> GSHMARENEMDENLEQVSGIIGNLRHMALDMGNEIDTQNRQIDRIMEKADSNKTRIDEANQRA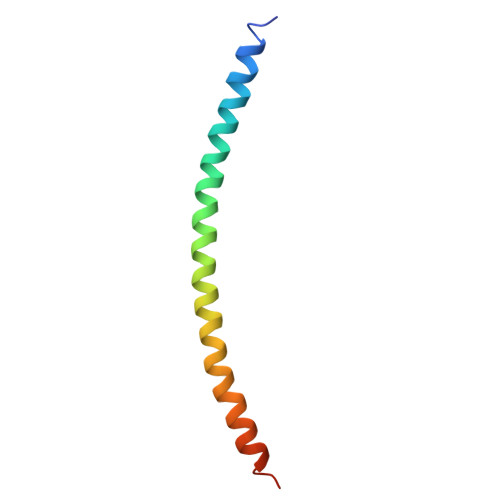TKMLG>[4x]GSHMLNIQNYSASPHPGIVAERPQTPSASEHVETAVVPSTTEHRGTDIISLSQAATKIHQAQQTLQSTPPISEEN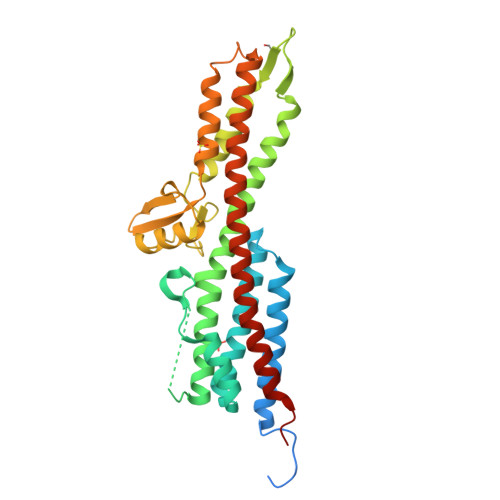NDERTLARQQLTSSLNALAKSGVSLSAEQNENLRSAFSAPTSALFSASPMAQPRTTISDAEIWDMVSQNISAIGDSYLGVYENVVAVYTDFYQAFSDILSKMGGWLLPGKDGNTVKLDVTSLKNDLNSLVNKYNQINSNTVLFPAQSGSGVKVATEAEARQWLSELNLPNSCLKSYGSGYVVTVDLTPLQKMVQDIDGLGAPGKDSKLEMDNAKYQAWQSGFKAQEENMKTTLQTLTQKYSNANSLYDNLVKVLSSTISSSLETAKSFLQG> HPETLVKVKDAEDQLGARVGYIELDLNSGKILESFRSEERFPMMSTFKVLLCGAILSRIDAGQEQLGRRIHYSQNDLVEYSPVTE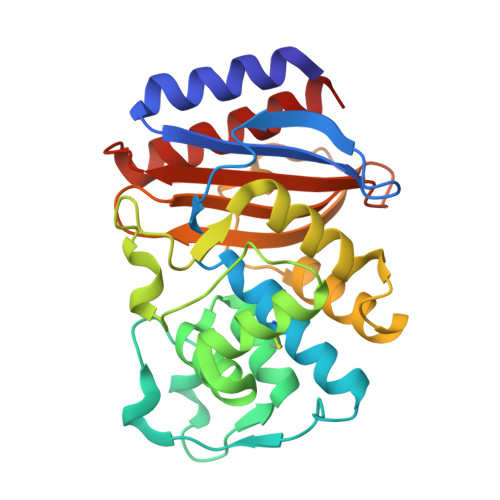KHLTDGMTVRELCSAAITMSDNTAANLLLTTIGGPKGLTAFLHNMGDHVTRLDRWEPELNEAIPNDERDTTTPVAMATTLRKLLTGELLTPASRQQLMDWMEADKVAGPLLRSVLPAGWFIADKSGAGERGSRGIVAALGPDGKPSRIVVIYTTGSQATMDELNRQIAEIGASLIKHW> SNAMSTLRLKEAKVPSVQFVGDDDV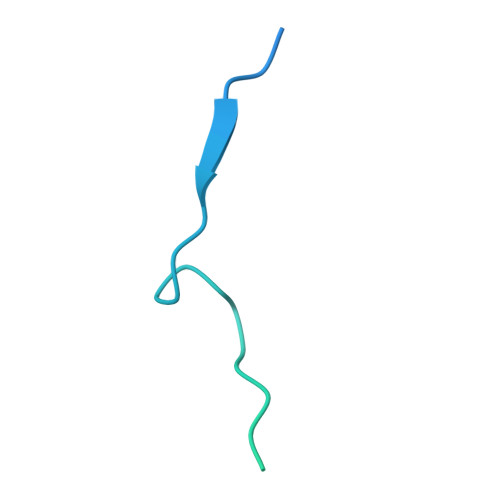LSHILDREGGTKLKKEKVQLLVNPQKVIKKAECELEKSDLEVLEDQNYVEVLGRNIQESLGNGSAVDGRNKVYSFQHR> MEEDDNLKKGNERNKKKAIFSNDDFTGEDSLMEDHLELREKLSEDIDMIKTSLKNNLVCSTLNDNEILTLSNYMQFFVFKSGNLVIKQGEKGSYFFIINSGKFDVYVNDKKVKTMGKGSSFGEAALIHNTQRSATIIAETDGTLWGVQRSTFRATLKQLSNRNFNENRTFIDSVSVFDMLTEAQKNMITNACVIQNFKSGETIVKQGDYGDVLYILKEGKATVYINDEEIRVLEKGSYFGERALLYDEPRSATIIAKEPTACASICRKLLNIVLGNLQVVLFRNIMTEALQQSEIFKQFSGDQLNDLADTAIVRDYPANYNILHKDKVKSVKYIIVLEGKVELFLDDTSIGILSRGMSFGDQYVLNQKQPFKHTIKSLEVCKIALITETCLADCLGNNNIDASIDYNNKKSIIKKMYIFRYLTDKQCNLLIEAFRTTRYEEGDYIIQEGEVGSRFYIIKNGEVEIVKNKKRLRTLGKNDYFGERALLYDEPRTASVISKVNNVECWFVDKSVFLQIIQGPMLAHLEERIKMQDTKVEMDELETERIIGRGTFGTVKLVHHKPTKIRYALKCVSKRSIINLNQQNNIKLEREITAENDHPFIIRLVRTFKDSKYFYFLTELVTGGELYDAIRKLGLLSKSQAQFYLGSIILAIEYLHERNIVYRDLKPENILLDKQGYVKLIDFGCAKKVQGRAYTLVGTPHYMAPEVILGKGYGCTVDIWALGICLYEFICGPLPFGNDEEDQLEIFRDILTGQLTFPDYVTDTDSINLMKRLLCRLPQGRIGCSINGFKDIKDHPFFSNFNWDKLAGRLLDPPLVSKSETYAEDIDIKQIEEEDAEDDEEPLNDEDNWDIDF

Previous work has demonstrated that one particular kinase, known as cyclic guanosine-3′,5′-monophosphate (cGMP)-dependent protein kinase, or protein kinase G (PKG), has essential roles in multiple stages of the parasite life cycle. Selective pharmacological inhibition of Plasmodium falciparum PKG (PfPKG) blocks the egress of merozoites and gametes from erythrocytes, as well as inhibits the motility of ookinetes in the mosquito and invasion of hepatocytes by sporozoites. The cellular functions of parasite PKG are regulated by allosteric and cooperative binding of cGMP, similarly to how mammalian PKG is activated. In contrast, PKG enzymes of Plasmodium and other apicomplexan parasites have an extended N-terminal domain that features four CNBs upstream of the KD and are monomeric, resulting in an effective regulatory stoichiometry of 4:1.

Here, we describe the complete atomic structure of PKG from two human malaria parasite species, P. falciparum and Plasmodium vivax. In the Plasmodium PKG crystal structures, each protomer in the dimers can be described as four CNBs, which, together with the N lobe of the KD, form a pentagonal arrangement, with the KD C lobe locked in the center. CNB-A and -B make direct contact with and constrain (and are constrained by) the C lobe of the KD from functionally essential movement, resulting in a substructure of these three domains that closely resembles the R-C heterodimer of PKA. Interestingly, all three Plasmodium structures display a swapped domain arrangement, in which the N terminus of each protomer in the dimer interacts with the active site of the other. Similar to PKA, the KD of PfPKG adopts a classical bilobal structure flanked by an N-terminal helix (αAK) and a C terminus. Despite being locked in an overall autoinhibited state, PfPKG–KD surprisingly exhibits many structural features of an active kinase, including: (i) interaction between the catalytic lysine K570 and E589 (on helix αCK); (ii) positioning of the helix αCK toward the ATP-binding site; (iii) an open (active) conformation of the activation loop; and (iv) intact hydrophobic spines. ΑAK in PfPKG makes multiple contacts with the N and the C lobes, some of which involve R809 as well as the C terminus of PfPKG–KD, and none of which have been observed in PKA. The contact between the two termini features a salt bridge between R528 and D597 as well as a π-bond between H524 and R809. In site 1, the basic AIS in PfPKG is docked against the activation loop of the KD in a manner reported for PKA, with key lysines (K15 and K16) replacing homologous arginines (R94 and R95 in PKAR–RIa) in interacting with the P+1 loop on the KD. The third CNB, pCNB-C, stands out because a hydrophobic network consisting of Y363, H373, F371, and F359 occludes the cGMP-binding pocket.(5E)-3-butyl-5-[(4-hydroxyphenyl)methylidene]-2-sulfanylidene-1,3-thiazolidin-4-one | C14 H15 N O2 S2 | 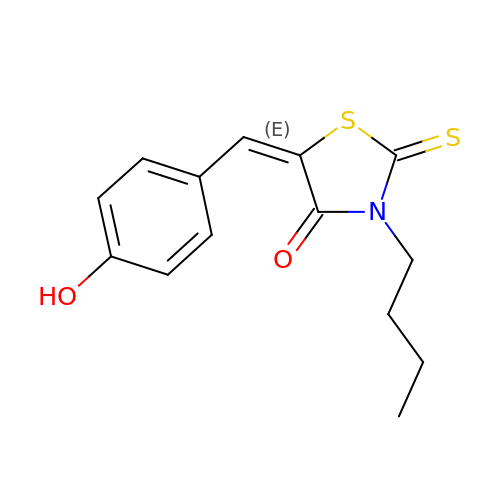WYSQOCWIYDTTJF-FMIVXFBMSA-N>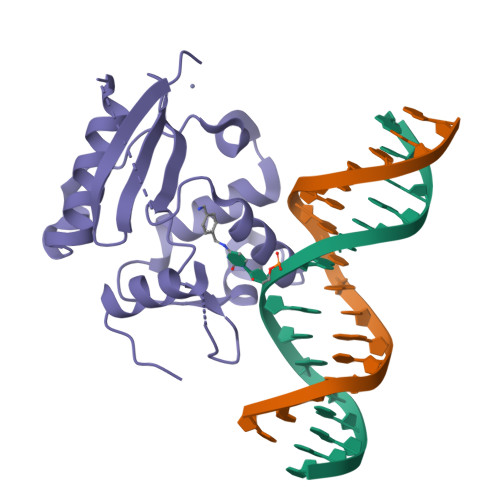[3x]MDKDCEMKRTTLDSPLGKLELSGCEQGLHEIKLLGKGTSAADAVEVPAPAAVLGGPEPLMQCTAWLNAYFHQPEAIEEFPVPALHHPVFQQESFTRQVLWKLLKVVKFGEVISYQQLAALAGNPKAARAVGGAMRGNPVPILIPCHRVVCSSGAVGNYSGGLAVKEWLLAHEGHRLGKP>[2x]RQSVCAGTENKLSSLSDLEQQYRALRKYYENCEVVMGNLEITSIEHNRDLSFLRSVREVTGYVLVALNQFRYLPLENLRIIRGTKLYEDRYALAIFLNYRKDGNFGLQELGLKNLTEILNGGVYVDQNKFLCYADTIHWQDIVRNPWPSNLTLVSTNGSSGCGRCHKSCT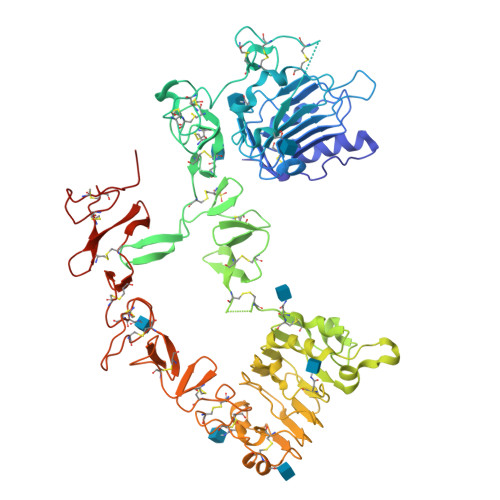GRCWGPTENHCQTLTRTVCAEQCDGRCYGPYVSDCCHRECAGGCSGPKDTDCFACMNFNDSGACVTQCPQTFVYNPTTFQLEHNFNAKYTYGAFCVKKCPHNFVVDSSSCVRACPSSKMEVEENGIKMCKPCTDICPKACDGIGTGSLMSAQTVDSSNIDKFINCTKINGNLIFLVTGIHGDPYNAIEAIDPEKLNVFRTVREITGFLNIQSWPPNMTDFSVFSNLVTIGGRVLYSGLSLLILKQQGITSLQFQSLKEISAGNIYITDNSNLCYYHTINWTTLFSTINQRIVIRDNRKAENCTAEGMVCNHLCSSDGCWGPGPDQCLSCRRFSRGRICIESCNLYDGEFREFENDSICVECDPQCEKMEDGLLTCHGPGPDNCTKCSHFKDGPNCVEKCPDGLQGANSFIFKYADPDRECHPCHPNCTQGCNGPTSHDCIYYPWTGH>TSEEPPFDIRALRADIEDMISEKLELGPSLIRLAWHEAASYDCFK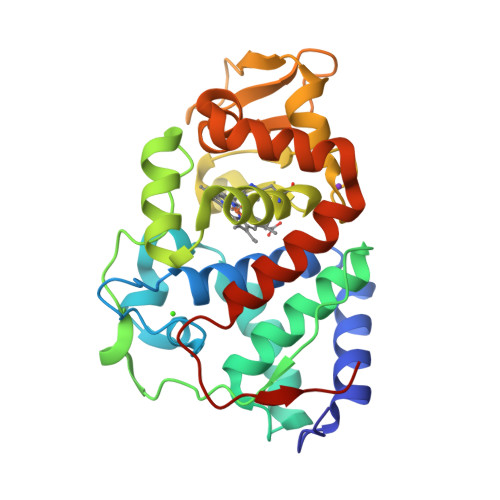KDGSPNSASMRFKPECLYAGNKGLDIPRKALETLKKKYPQISYADLWVLAAYVAIEYMGGPTIPFCWGRVDAKDGSVCGPDGRLPDGSKTQSHVREVFRRLGFNDQETVALIGAHTCGETHIEFSGYHGPWTHDKNGFDNSFFTQLLDEDWVLNPKVEQMQLMDRATTKLMMLPSDVCLLLDPSYRKYVELYAKDNDRFNKDFANAFKKLTELGTRNLHKAPASES[2x]> NRLSVKLPGLDLKNPIIPASGCFGFGEEYAKYYDLNKLGSIMVKATTLHPRFGNPTPRVAETASGMLNADGLQNPGLEVIMAEKLPWLNENFPDLPIIANVAGSEEDDYVAVCAKIGDAPNVKVIELNISCPNVKHGGQAFGTDPDVAAALVKACKAVSKVPLYV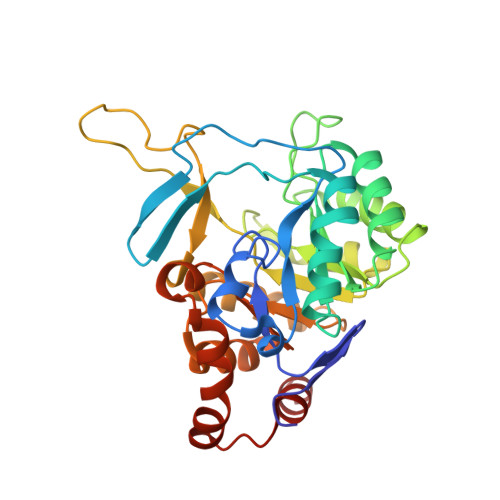KLSPNVTDIVPIAKAVEAAGADGLTMINTLMGVRFDLKTRKPVLANITGGLSGPAIKPVALKLIHQVAQVVDIPIIGMGGVESAQDVLEMYMAGASAVAVGTANFADPFVCPKIIEKLPEVMDQYGIDSLENLIQEVKNSK5-amino-1-(pyridin-4-yl)-1H-imidazole-4-carboxamide | C9 H9 N5 O | 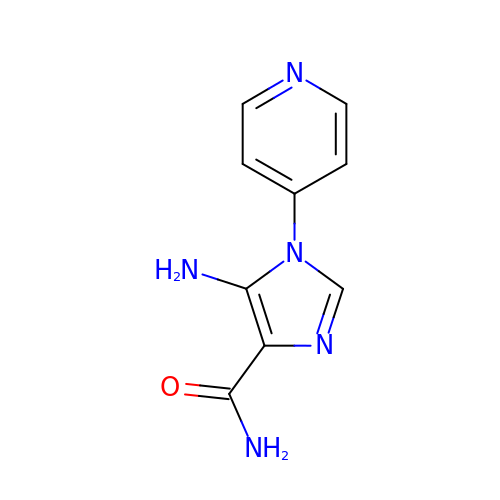JYYYJULWGCNUJZ-UHFFFAOYSA-N>GAVVGGLGGYMLGSAMSRP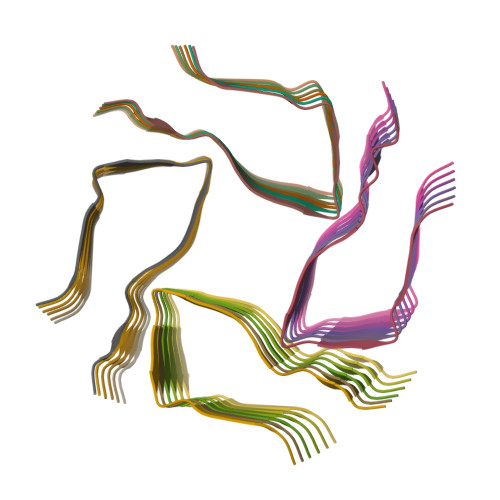MMHFGN[24x]> MPFMWRQRAYCAPVPSAFASQQPNGLGGEAGVRKPLLR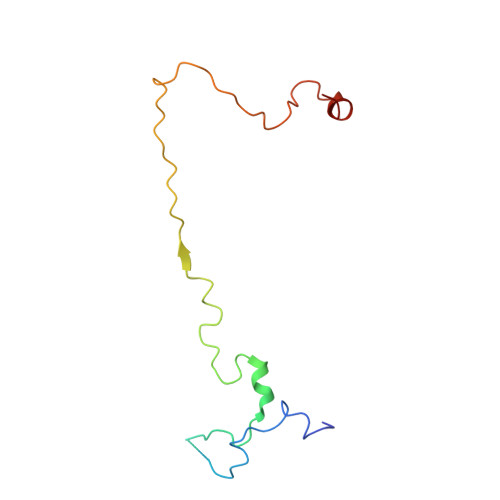SNSESLSVFSQIPDGLLGHTTSVTMGNSDIFFLPKPSNLLKIALPAFVFMPNLTIFTRAFPFYAHTSA>MNYPAEPFRIKSVETVSMIPRDERLKKMQEAGYNTFLLNSKDIYIDLLTDSGTNAMSDKQWAGMMMGDEAYAGSENFYHLERTVQELFGFKHIVPTHQGRGAENLLSQLAIKPGQYVAGNMYFTTTRYHQEKNGAVFVDIVRDEAHDAGLNIAFKGDIDLKKLQKLIDEKGAENIAYICLAVTVNLAGGQPVSMANMRAVRELTEAHGIKVFYDATRCVENAYFIKEQEQGFENKSIAEIVHEMFSYADGCTMSGKKDCLVNIGGFLCMNDDEMFSSAKELVVVYEGMPSYGGLAGRDMEAMAIGLREAMQYEYIEHRVKQVRYLGDKLKAAGVPIVEPVGGHAVFLDARRFCEHLTQDEFPAQSLAASIYVETGVRSMERGIISAGRNNVTGEHHRPKLETVRLTIPRRVYTYAHMDVVADGIIKLYQHKEDIRGLKFIYEPKQ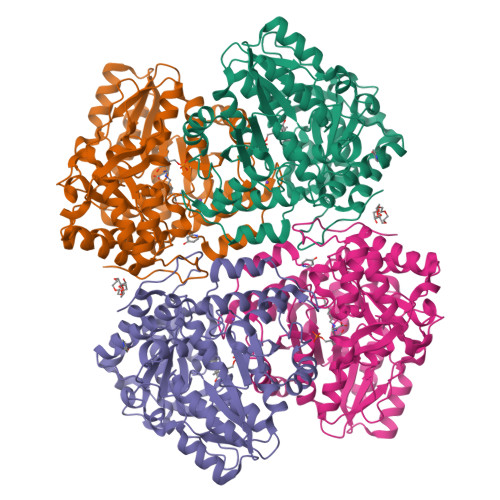LRFFTARFDYI[2x]[(2R,3S,4R,5R)-5-(6-amino-9H-purin-9-yl)-4-hydroxy-3-(phosphonooxy)oxolan-2-yl]methyl (3R)-4-({3-[(2-{[(1S)-1-{[(2R,3S,4S,5R,6R)-4,5-dihydroxy-6-{[(R)-hydroxy{[(R)-hydroxy{[(2R,3S,5R)-3-hydroxy-5-(5-methyl-2,4-dioxo-3,4-dihydropyrimidin-1(2H)-yl)oxolan-2-yl]methoxy}phosphoryl]oxy}phosphoryl]oxy}-2-methyloxan-3-yl]amino}ethyl]sulfanyl}ethyl)amino]-3-oxopropyl}amino)-3-hydroxy-2,2-dimethyl-4-oxobutyl 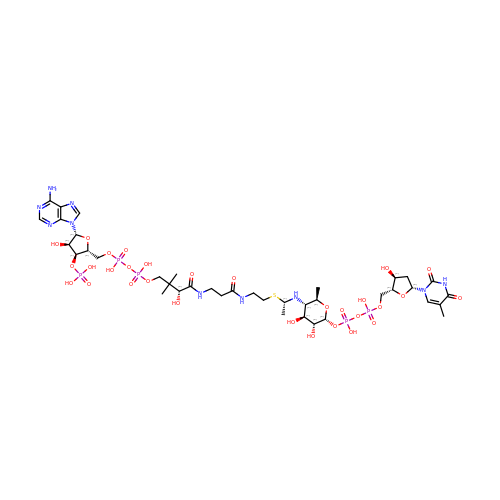dihydrogen diphosphate (non-preferred name) | C39 H65 N10 O30 P5 S | CAIUZPLIIIAOAA-MGECECIFSA-N N-[2-(2-{[(4R)-6-chloro-2-cyanoindolizin-8-yl]oxy}phenoxy)ethyl]-N-methylpropanamide 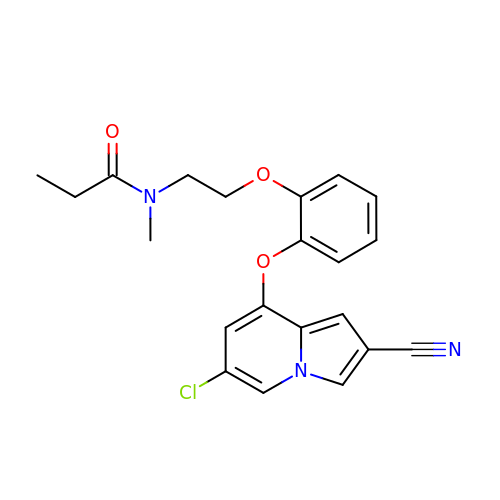| C21 H20 Cl N3 O3 | OANNJTAOFACLCJ-UHFFFAOYSA-N>[2x]SASEEQVAQD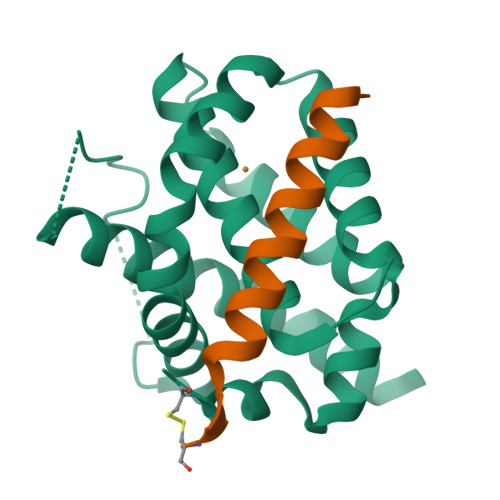TEEVFRSYVFYRHQQEQEAEGVAAPADPEMVTLPLQPSSTMGQVGRQLAIIGDDINRRYDSEFQTMLQHLQPTAENAYEYFTKIATSLFESGINWGRVVALLGFGYRLALHVYQHGLTGFLGQVTRFVVDFMLHHSIARWIAQRGGWVAALNLCNG;>EDIIRNIARHLAQMGDSMDRSWGGC[2x]>GPSGMILKRAYDVTPQKISTDKVRGVRKRVLIGLKDAPNFVMRLFTVEPGGLIDRHSHPWEHEIFVLKGKLTVLKEQGEETVEEGFYIFV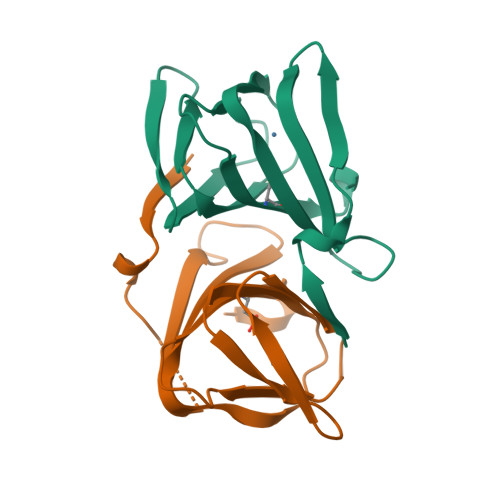EPNEIHGFRNDTDSEVEFLCLIPKEGGE[4x]>[2x]APKNELVQKFQVYYLGNVPVAKPVGVDVINGALESVLSSSSREQWTPSHVSVAPATLTILHQQTEAVLGECRVRFLSFLAVGRDVHTFAFIMAAGPASF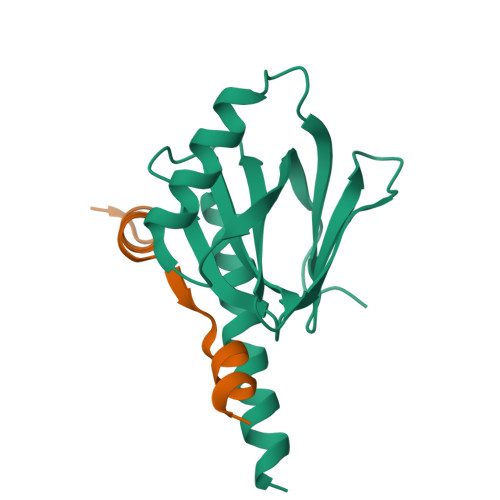CCHMFWCEPNAASLSEAVQAACMLRYQKCLDARSQHHHHHH;>GAMDAAVEPEERHLSKMQQNGYENPTYKFFEQMQN[2x]> AGVMTGAKFTQIQFGMTRQQVLDIAGAENCETGGSFGDSIHCRGHAAGDY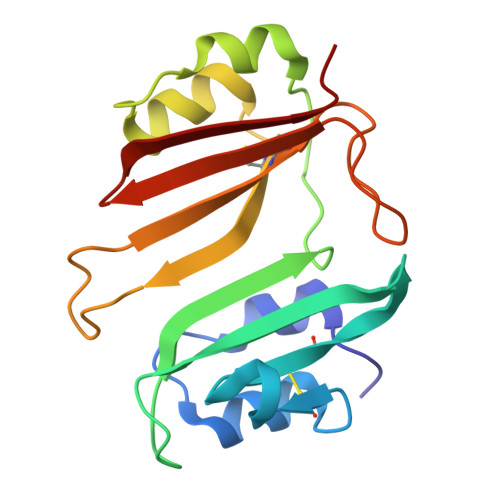YAYATFGFTSAAADAKVDSKSQEALLAPSAPTLTLAKFNQVTVGMTRAQVLATVGQGSCTTWSEYYPAYPSTAGVTLSLSCFDVDGYSSTGAARGSAHLWFTDGVLQGKRQWDLV> GSKGLENPLPERPREKEEPVVRETGEVVDCHLSDMLQQLHSVNASKPSERGLVRQEEAEDPACIPIFWVSKWVDYSDKYGLGYQLCDNSVGVLFNDSTRLILYNDGDSLQYIERDGTESYLTVSSHPNSLMKKITLLKYFRNYMSEHLLKAGANITPREGDELARLPYLRTWFR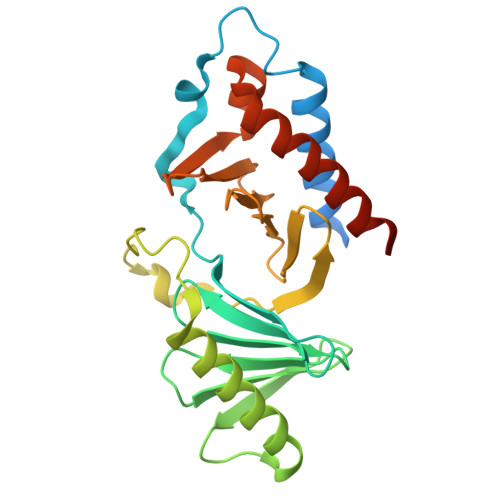TRSAIILHLSNGSVQINFFQDHTKLILCPLMAAVTYIDEKRDFRTYRLSLLEEYGCCKELASRLRYARTMVDKLLSSRSASNRLKAS>[4x]GPMVSEQSEIVTSKYQKIAVAVAQRIANGDYEVGEKLKSRTTIASTFNVSPETARKGLNILADLQILTLKHGSGAIILSKEKAIEFLNQYETSHSVAILKGKIRDNIKAQQQEMEELATLVDDFLLQTRAVSKQYPLAPYEIIVSEDSEHLGKSIGELNVWHQTGATIVAIEHEGKFIVSPGPFSVIEQGDHIFFVGDEDVYARMKTYFNLRMGL

BusR is a member of a yet structurally uncharacterized subfamily of the GntR family of transcription factors that downregulates transcription of the genes for the BusA (OpuA) glycine-betaine transporter upon c-di-AMP binding. BusR satisfies the overall domain architecture of the GntR family with its N-terminal winged helix-turn-helix motif (wHTH) and a C-terminal effector binding motif, an RCK_C domain (regulator of K+ conductance). Our structural data, supported by biochemical and biophysical data, reveal that BusR utilizes a unique domain assembly with a tetrameric coiled-coil in between the binding platforms, serving as a molecular ruler to specifically recognize a 22 bp separated bipartite binding motif. Binding of c-di-AMP to BusR induces a shift in equilibrium from an inactivated towards an activated state that allows BusR to bind the target DNA, leading to transcriptional repression.

In order to understand the molecular mechanisms of BusR signaling we crystallized selenomethionine substituted full-length BusR and solved its structure to 2.8 Å resolution by single-wavelength anomalous diffraction experiment. As the protein was recombinantly expressed and purified from E. coli, that lack DAC domain proteins and the entire c-di-AMP pathway, our structure represents the apo state. The asymmetric unit contains the physiological functional tetramer of BusR. The four central αCC-helices of the four monomers constitute a four-stranded coiled-coil motif, thereby forming a robust tetramerization interface. The four monomers are arranged in a 2-parallel 2-antiparallel head-to-tail arrangement, forming an overall shape resembling a dumbbell. The RCK_C domains form a dimer on each side of the BusR dumbbell. Each of these dimers is flanked by the two wHTH motifs of the antiparallel strands. The interfaces between the RCK_C dimer and its neighbouring wHTH motifs differ significantly resulting in two distinct DNA binding domain arrangements that we refer to as wHTHinhib and wHTHfree. The interface between the RCK_C domain and wHTHinhib is approx. 50% larger in buried surface area (wHTHfree: area = 902 Å2 versus wHTHinhib: area = 1353 Å2). Furthermore, in the observed conformation, the DNA recognition helix αG3 of wHTHinhib is buried in the interface and thus incapable to bind to DNA.> MNIEKVILDWNEYIEAARSVVSEGCVLLENNGTLPLEKGAVVSIFGRIQTHYYKSGTGSGGMVNVTHVVGVPEGLKLSEHVTVNEELENIYKEWEEENPFDEGLGWGTEPWSQPEMELTDEIVSNASAKSDVAIVIIGRTAGEDKDFSDVAGAYKLSETEEDMLRRVRKHFDKMVVLLNVGSLMDLNVISEINPDALMVIWQGGMIGGLGTADVLTGKVNPSGKLTDTIAYEINDYPSTENFGDPVRDYYAEDIYVGYRYFETFEKSKVRYPFGYGISYTEFEHTVGEFTADINSRTFTASCTVKNTGSVAGKDVAQFYVSAPQGKLGKPEKVLVAFKKTGILNPGKEEKITVTVPFDRFASFDDTGVTGAESCFVLEAGEYTVYEGKNVRESYKEGSFTLEENIVTEKLSKALAPMESFKRMKASENSDGTLSVKYEDVPVSDVDEKKRRLDNMPVEIPQDFTARYSLKDVLSGSVDMEKFIARLSDDDLACIVRGEGMGSSLVTAGTAAAFGGVSEYLRKMDIPAVCCDDGPSGMRLDSGATAFSMPNGTMLASTFNPDVIERMYGFTSLEMIYNKVECLLGPGMNIHRNPL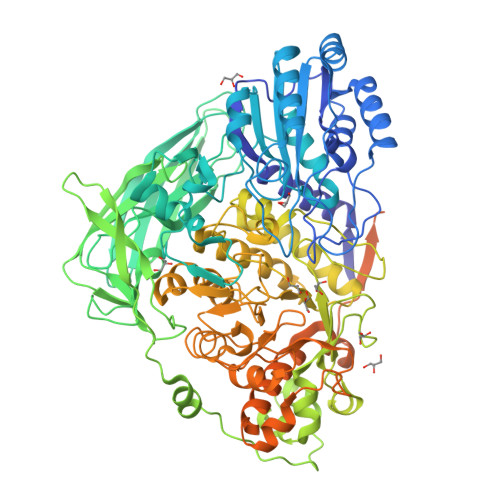NGRNFEYFSEDPYLNGTIASAMLKGLHKYGSDGVAKHFCCNNQELGRQACDSVVSQRALREIYLKGFEIAVKEGGCKAFMTTYAQVNGMWTAGNYDLNTRILRDEWGFKGIVMTDWWAQVNDRGGEPTKNNTAAMVRAQNDLYMVTANAAMNSANDNTLSQLSEGKLNRAELQRCAMNICEYAMNTMAMKRLCRNDIKVEIAGRVIEEDAFDIENAEYLVLKGNITVSLKNKESKAGTNYYIPLDIQDLGMYDISVTASSMLGEVAQLPCTLYYTGVPFLTYTFNGSGGKDVTITKSMDFHNRMAVIRLNVAKNGLNLDRIEFKKQQ> ADTIVAVELDSYPNTDIGDPNYPHIGIDIKSIRSKSTARWNMQTGKVGTVGISYNSVAKRLSAVVSYSGSSSTTVSYDVDLNNVLPEWVRVGLSATTGLYKETNTILSWSFTSKLKTNSIADENSLHFSFNKFSQNPKDLILQGDAFTDSDGNLQLTKVSSSGDPQGNS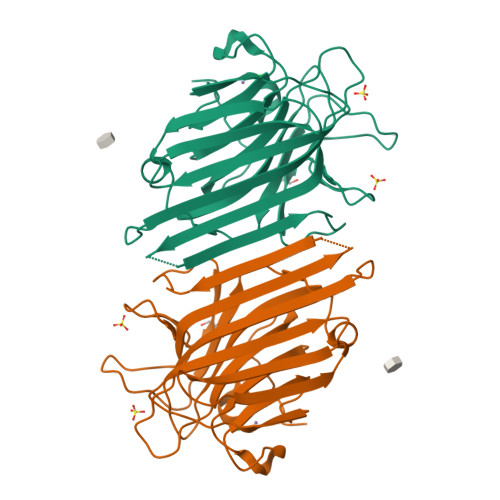VGRALFYAPVHIWEKSAVVASFDATFTFLIKSPDREPADGITFFIANTDTSIPSGSGGRLLGLFPDAN> GSSSWNDIKNSGYISRYLTDFEPIQCLGRGGFGVVFEAKNKVDDCNYAIKRIRLPNRELAREKVMREVKALAKLEHPGIVRYFNAWLEAPPEKWQEKLQPSSPKVYLYIQMQLCRKENLKDWMNGRCTIEERERSVCLHIFLQIAEAVEFLHSKGLMHRNLKPS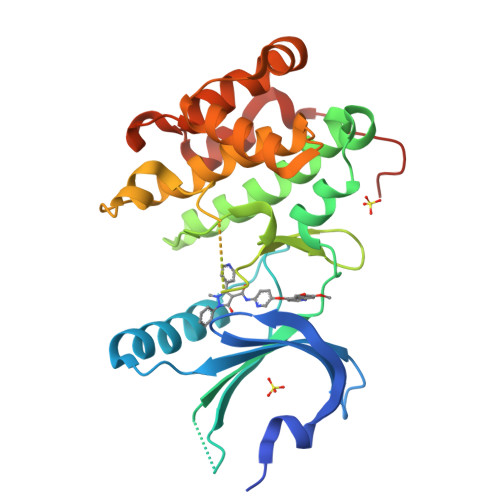NIFFTMDDVVKVGDFGLVTAMDQDEEEQTVLTPMPAYARHTGQVGTKLYMSPEQIHGNSYSHKVDIFSLGLILFELLYPFSTQMERVRTLTDVRNLKFPPLFTQKYPCEYVMVQDMLSPSPMERPEAINIIENAVFEDLDFPGKTVLRQRSRS> MRAGCVACSRIPKLGIAALGSTTTSMQATCQETQELRCATTQMAPAVIFPLPPPLRGSYIDRKPTAASFNEHHAT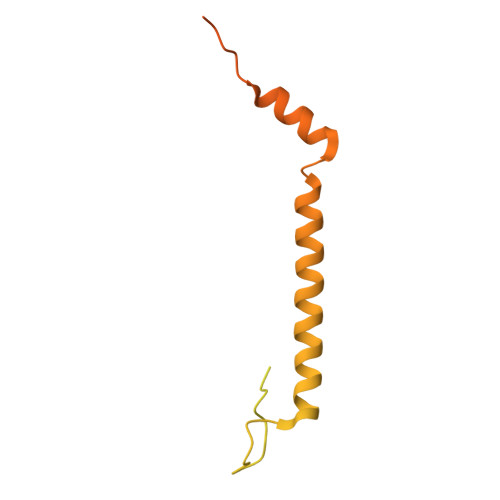ASFRHHMIASADVSHRPRHFYFASGTRNDTGTRSVKEGERKQLKQQTNVEVDSVAYGDQLDELSARWAAKFYGQVTFGPRNYPYPSSRWLARRFQMKKHRIIKRFRFRRYKLAAVANLPFAKMIRVGMLPELKSSKTKRGDVVDPTLSGQLVSAVKNTGEKRKGQRTRPKSKYQV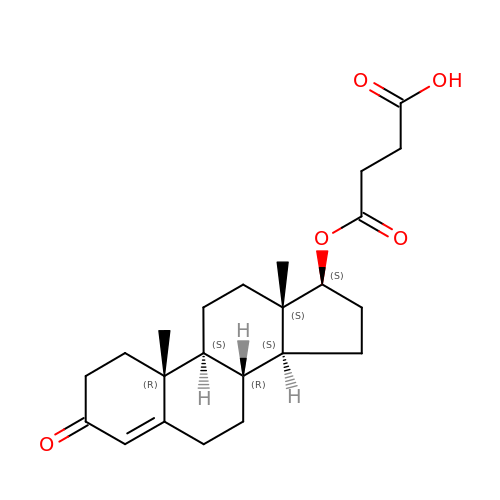TESTOSTERONE HEMISUCCINATE | C23 H32 O5 | CJQNBXFUHQZFOE-VYAQIDIUSA-N>CCCCGGTACCGG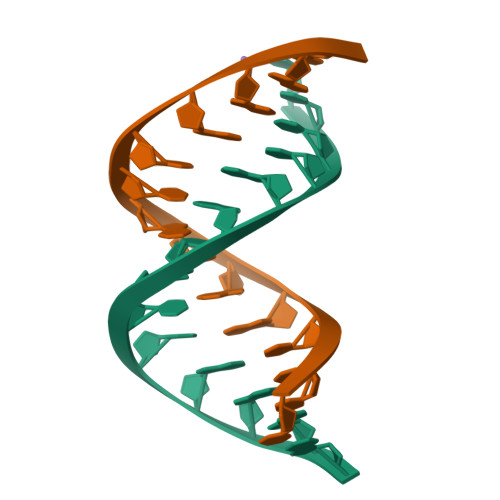GG[2x]>MTKTLPKDFIFGGATAAYQAEGATHTDGKGPVAWDKYLEDNYWYTAEPASDFYHKYPVDLELAEEYGVNGIRISIAWSRIFPTGYGEVNEKGVEFYHKLFAECHKRHVEPFVTLHHFDTPEALHSNGDFLNRENIEHFIDYAAFCFEEFPEVNYWTTFNEIGPIGDGQYLVGKFPPGIKYDLAKVFQSHHNMMVSHARAVKLYKDKGYKGEIGVVHALPTKYPYDPENPADVRAAELEDIIHNKFILDATYLGHYSDKTMEGVNHILAENGGELDLRDEDFQALDAAKDLNDFLGINYYMSDWMQAFDGETEIIHNGKGEKGSSKYQIKGVGRRVAPDYVPRTDWDWIIYPEGLYDQIMRVKNDYPNYKKIYITENGLGYK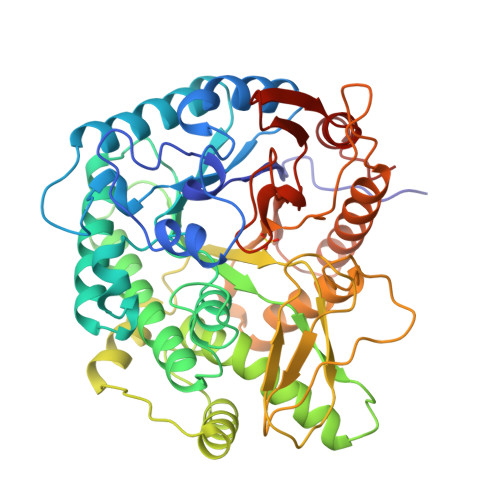DEFVDNTVYDDGRIDYVKQHLEVLSDAIADGANVKGYFIWSLMDVFSWSNGYEKRYGLFYVDFDTQERYPKKSAHWYKKLAETQVIE[2x]Human bestrophin1 (hBest1) is a Ca2+-activated Cl− channel essential for Cl− transport in retinal pigment epithelium (RPE). Although the structure of hBest1 is still unsolved, two Best1 homolog structures, one from bacteria Klebsiella pneumoniae (KpBest) and the other from chicken (cBest1), have been previously reported. Overall, the channel is a pentameric assembly with a single ion-conducting pathway, which varies in diameter along its length and is constrained at two narrow points: a “neck” contributed by three residues (I62/I66/F70 in KpBest and I76/F80/F84 in hBest1/cBest1) on a transmembrane helix, and an “aperture” formed by a single residue (I180 in KpBest1, I205 in hBest1, and V205 in cBest1) on a cytosolic helix. Here, by electrophysiological and structural analyses, we show that the neck and aperture in hBest1 are both indispensable Ca2+-dependent gates, and their dysregulated opening by rationally designed or patient-derived mutations causes Ca2+-independent leak and elevates Ca2+-dependent channel activity.

Alanine substitution mutants for each of the 12 residues were generated in KpBest and hBest1 and subjected to crystallography and patch clamp, respectively. Moreover, the equivalent KpBest mutants (W16A, G18A, S19A, L259A, P262A, G264A, and D269A) all showed an overall similar structure to that of WT KpBest. The corresponding “Ca2+-binding” sites in WT KpBest are occupied by Zn2+, an essential component in the crystallization buffer. Notably, the short extracellular domains of hBest1 represent a challenge for quantitative measurement of the surface expression by labeling techniques (e.g., biotin). They can be classified into three groups by different molecular mechanisms: (1) mutations on residues involved in Ca2+ binding, including W24A, G26A, S27A, L294A, P297A, F298A, G299A, and D304A, likely cause defects of Ca2+-dependent activation; (2) mutations at the neck/aperture, including I205A, I205T, 3A, and 4A, increase open probability by functionally mimicking a constant open state; and (3) mutations outside of the neck/aperture, including D203A, P233A, Y236A, Y236C, W287A, and W287F, alter open probability through the neck/aperture residues.

>[5x]SNAMIIRPEQHWFLRLFDWHASVLSKIIFRLLLNVLMSIIAIISYQWYEQLGIHLTVAPFSLLGIAIAIFLGFRNSASYSRFVEARNLWGTVLIAERTLVRQLRNILPAEHDAHRRIVSYLVAFSWSLKHQLRKTDPTADLRRLLPEERVTEILASSMPTNRILLLAGNEIGQLREAGKLSDITYGLMDNKLDELAHVLGGCERLATTPVPFAYTLILQRTVYLFCTLLPFALVGDLHYMTPFVSVFISYTFLSWDSLAEELEDPFGTAANDLPLNAMCNTIERNLLDMTGQHPLPE> GSHMIEGYECQPIFLNVLEAIEPGVVCAGHDNNQPDSFAALLSSLNELGERQLVHVVKWAKALPGFRNLHVDDQMAVIQYSWMGLMVFAMGWRSFTNVNSRMLYFAPDLVFNEYRMHKSRMYSQCVRMRHLSQEFGWLQITPQEFLCMKALLLFSIIPVDGLKNQKFFDELRMNYIKELDRIIACKRKNPTSCSRRFYQLTKLLDSVQPIARELHQFAFDLLIKSHMVSVDFPEMMAEIISVQVPKILSGKVKP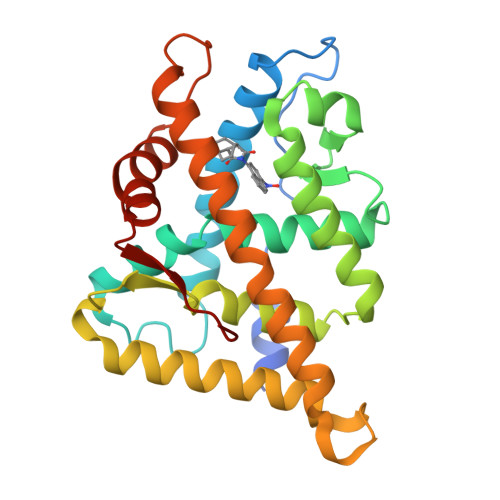IYFHTQ>TEKFDFGTMVQWAYDHKYAEESKIAYEYALAAGSDSNARAFLATNSQAKHVKDCATMVRHYLRAETQALSMPAYIKARCKLATGEGSWKSILTFFNYQNIELITFINALKLWLKGIPKKNCLAFIGPPNTGKSMLCNSLIHFLGGSVLSFANHKSHFWLASLADTRAALVDDATHACWRYFDTYLRNALDGYPVSIDRKHKAAVQIKAPPLLVTSNIDVQAEDRYLYLHSRVQTFRFEQPCTDESGEQPFNITDADWKSFFVRLWGRLDLIDEEEDSEEDGDSMRTFTCSARNTNAVD[6x];>GSRATVFKLGLFKSLFLCSFHDITRLFKNDKTTNQQWVLAVFGLAEVFFEASFELLKKQCSFLQMQKRSHEGGTCAVYLICFNTAKSRETVRNLMANMLNVREECLMLQPPKIRGLSAA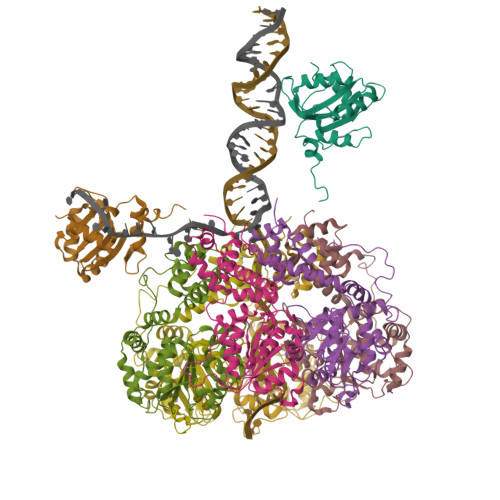LFWFKSSLSPATLKHGALPEWIRAQTTLNAAAA[2x]>EDAALREEAKGLFEVIPMQAPQLADNNTVTRDKIDLGAMLFFDPRMSKSGVFSCQSCHNVGLGGVDGLETSIGHGWQKGPRNAPTALNAVFNVAQFWDGRAPDLAAQAKGPVQAGVEMNNTPENLVATVQSMPGYVEAFAKAFPGQKDPISFDNFALAVEAFE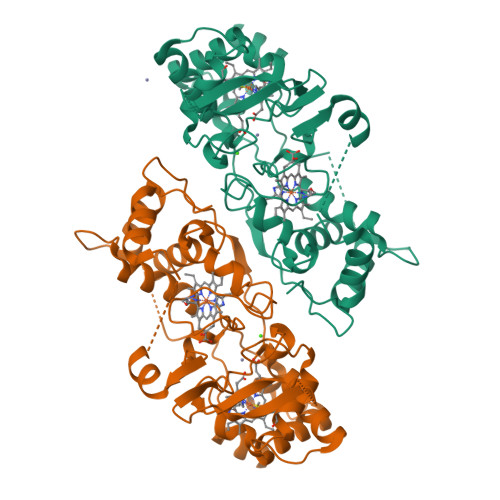ATLITPNSKFDQWLMGADGAMSADEKAGLKLFIDTGCAACHNGINIGGNGYYPFGVVEKPGAEVLPAGDKGRFAVTATADDEYVFRAGPLRNIALTAPYFHSGKVWDLREAVSVMANSQLGATLDDTQVDQITAFLGTLTGEQPEVVHPILPVRSAQTPRPEHMN[4x]> AQSVPWGISRVQAPAAHNRGLTGSGVKVAVLDTGISTHPDLNIRGGASFVPGEPSTQDGNGHGTHVAGTIAALDNSIGVLGVAPSAELYAVKVLGASGSGAISSIA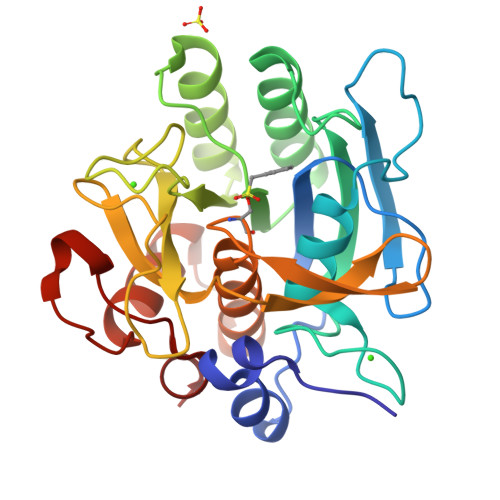QGLEWAGNNGMHVANLSLGSPSPSATLEQAVNSATSRGVLVVAASGNSGAGSISYPARYANAMAVGATDQNNNRASFSQYGAGLDIVAPGVNVQSTYPGSTYASLNGTSMATPHVAGAAALVKQKNPSWSNVQIRNHLKNTATSLGSTNLYGSGLVNAEAATR> MAHHHHHHMSPADAVGQIRQNATQVLTILKSGDAASARPKAEAYAVPYFDFQRMTALAVGNPWRTASDAQKQALAKEFQTLLIRTYSGTMLKFKNATVNVKDNPIVNKGGKEIVVRAEVGIPG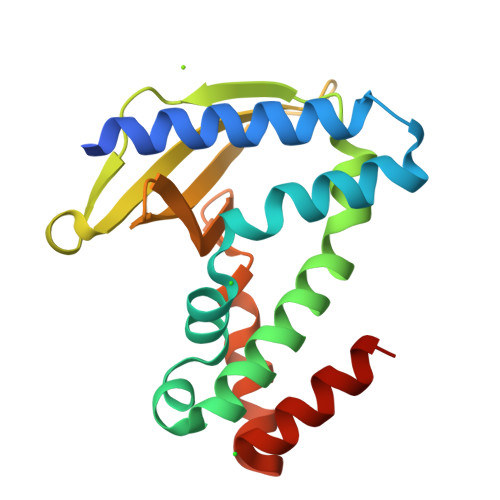QKPVNMDFTTYQSGGKYRTYNVAIEGTSLVTVYRNQFGEIIKAKGIDGLIAELKAKNGGK>[8x]MSVSAFNRRWAAVILEAL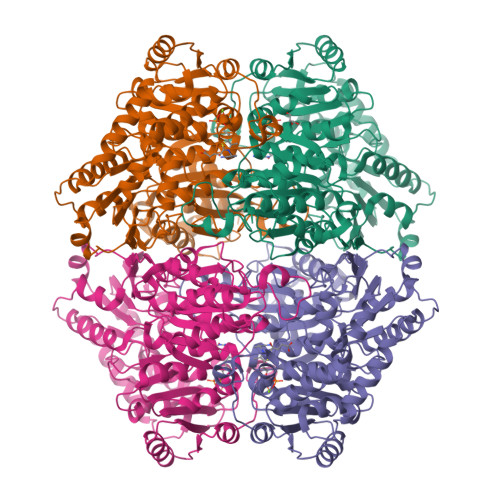TRHGVRHICIAPGSRSTPLTLAAAENSAFIHHTHFDERGLGHLALGLAKVSKQPVAVIVTSGTAVANLYPALIEAGLTGEKLILLTADRPPELIDCGANQAIRQPGMFASHPTHSISLPRPTQDIPARWLVSTIDHALGTLHAGGVHINCPFAEPLYGEMDDTGLSWQQRLGDWWQDDKPWLREAPRLESEKQRDWFFWRQKRGVVVAGRMSAEEGKKVALWAQTLGWPLIGDVLSQTGQPLPCADLWLGNAKATSELQQAQIVVQLGSSLTGKRLLQWQASCEPEEYWIVDDIEGRLDPAHHRGRRLIANIADWLELHPAEKRQPWCVEIPRLAEQAMQAVIARRDAFGEAQLAHRICDYLPEQGQLFVGNSLVVKLIDALSQLPAGYPVYSNRGASGIDGLLSTAAGVQRASGKPTLAIVGDLSALYDLNALALLRQVSAPLVLIVVNNNGGQIFSLLPTPQSERERFYLMPQNVHFEHAAAMFELKYHRPQNWQELETAFADAWRTPTTTVIEMVVNDTDGAQTLQQLLAQVSHL> GMTILSDVKALGQQIWLDNLSRSLVQSGELAQMLKQGVCGVTSNPAIFQKAFAGDALYADEVAALKRQNLSPKQRYETMAVADVRAACDVCLAEHESTGGKTGFVSLEVSPELAKDAQGTVEEARRLHAAIARKNAMIKVPATDAGIDALETLVSDGISVNLTLLFSRAQTLKAYAAYARGIAKRLAAGQSVAHIQVVASFFISRVDSALDATLPDRLKGKTAIALAKAAYQDWEQYFTAPEFAALEAQGANRVQLLWASTGVKNPAYPDTLYVDSLIGVHTVNTVPDATLKA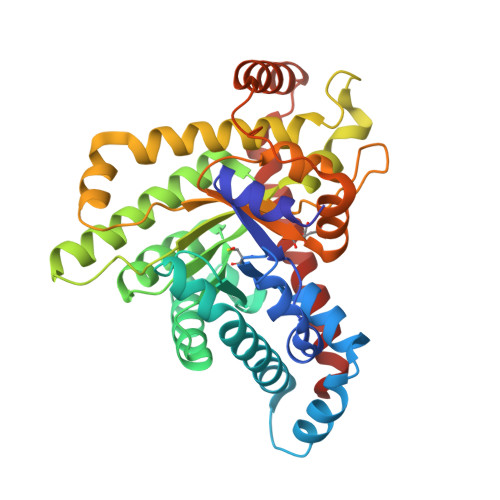FIDHGTAKATLTESADEARARLAEIAALGIDVETLAARLQEDGLKQFEEAFEKLLAPLV Anchoring of these surface proteins to the cell wall peptidoglycan requires transpeptidase enzymes called sortases, a product of an srt (surface protein sorting) gene. The membrane-associated sortase recognizes the LPXTG motif of the substrate protein, cleaves between the Thr and Gly, and forms an acyl-enzyme intermediate. According to the current model of sortase-mediated pilus assembly, the pilus polymerization catalyzed by a pilus-specific sortase is followed by cell wall anchoring of pilus polymers by the housekeeping sortase. To understand the molecular basis of pilin sorting and pilus anchoring within a bacterial strain, we investigated the housekeeping sortase, GBSSrtA, and a pilus-specific sortase, GBSSrtC1, from the PI-1 pathogenicity island of S. agalactiae SAG 2603 V/R. Either GBSSrtC1 or GBSSrtC2 of this GBS strain is capable of polymerizing GBS80, the pilus shaft of the GBS PI-1 pili.

Therefore, we generated a Cys184Ala mutant of GBSSrtC1, containing the lid mutation (KDPYS to IPNTG), and used this mutant for crystallization. The association of the two GBSSrtC1-lidM monomers observed in the triclinic unit cell, related by a non-crystallographic 2-fold axis, is identical to that observed for the type II and III GBSSrtC1 dimer association. The two monomers of GBSSrtC1-lidM, with an rmsd of 0.63 Å over 164 atoms, display differences around the active site region. Molecule A showed a continuous electron density for the hinge region between H2 and the lid, and this formed an extra helical turn. The lid in both chains was visible up to Leu47, which points inwards into the hydrophobic pocket, positioned precisely as in GBSSrtC1 structures. The low B factors for Leu47 in GBSSrtC1-lidM and its surrounding hydrophobic environment may suggest that the spatial disposition of Leu47 acts as an anchor to the lid. The disposition of Ala184 and the catalytic His122 and Arg193 remained unaffected in the absence of the DP(W/F/Y) motif; however, the orientation of Arg193 side chain was slightly different from that seen in the GBSSrtC1 structures. Because the DP(W/F/Y) motif was dislodged by mutation, the entire elongated groove was potentially available for binding; however, the active site is empty around the catalytic residues.

>[2x]MRGSHHHHHHGSSHANINAFKEAVTKIDRVEINRRLELAYAYNASIAGAKTNGEYPALIPNTGAEQKQAGVVEYARMLEVKEQIGHVIIPRINQDIPIYAGSAEENLQRGVGHLEGTSLPVGGESTHAVLTAHRGLPTAKLFTNLDKVTVGDRFYIEHIGGKIAYQVDQIKVIAPDQLEDLYVIQGEDHVTLLTATPYMINSHRLLVRGKRIPYVEKTVQKDSKTFRQQQ> GAMGAKVVIEPHRHAGVYIARGKEDLLVTKNMAPGESVYGEKRISVEEPSKEDGVPPTKVEYRVWNPFRSKLAAGIMGGLDELFIAPGKKVLYLGAASGTSVSHVSDVVGPEGVVYAVEFSHRPGRELISMAKKRPNIIPIIEDARHPQKYRMLIGMVDCVFADVAQPDQARIIALNSHMFLKDQGGVVISIKANCIDSTVDAETVFAREVQKLREERIKPLEQLTLEPYERDHCIVVGRYMRSGLKK;> GAMAPIEYLLFEEPTGYAVFKVKLQQDDIGSRLKEVQEQINDFGAFTKLIELVSFAPFKGAAEALENANDISEGL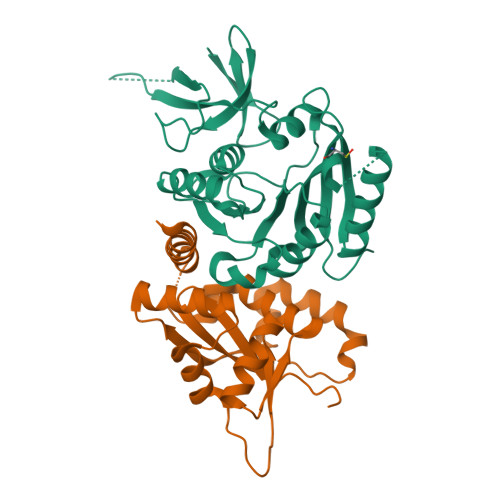VSESLKAILDLNLPKASSKKKNITLAISDKNLGPSIKEEFPYVDCISNELAQDLIRGVRLHGEKLFKGLQSGDLERAQLGLGHAYSRAKVKFS> GPMQQANLGDGVATARLLSRSDWGARLPKSVEHFQGPAPYVIIHHSYMPAVCYSTPDCMKSMRDMQDFHQLERGWNDIGFSFGIGGDGMIYTGRGFNVIGAHAPKYNDKSVGIVLIGDWRTELPPKQMLDAAKNLIAFGVFKGYIDPAYKLLGHRQVRDTECPGGRLFAEISSWPHFTHINDTEGVSSTTAPVVPHVHPQAAAPQKPHQSPPAAPKV

Drosophila PGRP-LB belongs to the amidase PGRPs and downregulates the immune deficiency (IMD) pathway by cleaving meso-2,6-diaminopimelic (meso-DAP or DAP)-type PGN. The structure of the PGRP domain comprises three α-helices and one central β-sheet composed of six β-strands, similar to the bacteriophage T7 lysozyme, a zinc-dependent amidase. The main difference between amidase and non-catalytic PGRPs is the presence of Zn2+ in only amidase PGRPs, which is coordinated by two histidines and one cysteine. We generated mutants to characterize the amidase reaction mechanism and solved the X-ray structures of wild-type Drosophila PGRP-LBPA/PC and its mutants in apo form or complexed to TCT.

To tackle these two scenarios, we designed and analyzed four different mutations of the conserved residues in the catalytic Drosophila PRGP-LBPA/PC: H42A, Y78F, H152A and C160S. Only the Y78F mutation caused complete loss of the enzymatic activity for every compounds. The introduced mutations did not affect the ability to recognize PGN, attesting that Y78 is the only residue taking part in the amidase mechanism. Initial X-ray and enzymatic analyses showed that the Y78F mutation does not destabilize the protein structure and prevents PGN substrate from being degraded. Y78F and C160S PGRP-LBPA/PC mutant structures were elucidated to 1.30 Å and 1.40 Å resolution, respectively. Both mutants Y78F and C160S PGRP-LBPA/PC share a similar fold with PGRP-LBPA/PC wild type with a RMSD on Cα of 0.49 Å and 1.12 Å, respectively, but in different space groups, P6122 for PGRP-LBPA/PC_Y78F and P1 for PGRP-LBPA/PC_C160S. PGRP-LBPA/PC_Y78F also presents a crystal packing artefact where E182 from the C-terminal of a symmetry-related molecule makes a coordination with Zn2+. By comparing the apo and complexed PGRP-LBPA/PC_Y78F structures, the C-terminal symmetry-related molecule is filling the binding pocket of the peptide moiety from the PGN attesting the non-physiological nature of this interaction. We showed that Zn2+ is totally absent in PGRP-LBPA/PC_C160S mutant as already observed in the structure resolution, while it is still present in PGRP-LBPA/PC_Y78A mutant and PGRP-LBPA/PC wild type. Regarding PGRP-LBPA/PC_Y78F, the amidase activity is also abolished without Zn2+ in the buffer.>MQRADSEQPSKRPRCDDSPRTPSNTPSAEADWSPGLELHPDYKTWGPEQVCSFLRRGGFEEPVLLKNIRENEITGALLPCLDESRFENLGVSSLGERKKLLSYIQRLVQIHVDTMKVINDPIHGHIELHPLLVRIIDTPQFQRLRYIKQLGGGYYVFPGASHNRFEHSLGVGYLAGCLVHALGEKQPELQISERDVLCVQIAGLCHDLGHGPFSHMFDGRFIPLARPEVKWTHEQGSVMMFEHLINSNGIKPVMEQYGLIPEEDICFIKEQIVGPLESPVEDSLWPYKGRPENKSFLYEIVSNKRNGIDVDKWDYFARDCHHLGIQNNFDYKRFIKFARVCEVDNELRICARDKEVGNLYDMFHTRNSLHRRAYQHKVGNIIDTMITDAFLKADDYIEITGAGGKKYRISTAIDDMEAYTKLTDNIFLEILYSTDPKLKDAREILKQIEYRNLFKYVGETQPTGQIKIKREDYESLPKEVASAKPKVLLDVKLKAEDFIVDVINMDYGMQEKNPIDHVSFYCKTAPNRAIRITKNQVSQLLPEKFAEQLIRVYCKKVDRKSLYAARQYFVQWCADRNFTKPQDGDVIAPLITPQKKEWNDSTSVQNPTRLREASKSRVQLFKDDPM[4x]

Sterile alpha motif and HD-domain containing protein 1 (SAMHD1) is a dNTP triphosphohydrolase that catalyses the breakdown of dNTPs to constituent 2′-deoxynucleoside and triphosphate, and is therefore an important regulator of cellular nucleotide homeostasis in mammalian cells. SAMHD1 dNTP triphosphohydrolase catalytic activity requires assembly into homo-tetramers. Sequences at the N- and C-termini of the HD domain stabilise inter-monomer protein-protein interactions and incorporate four pairs of allosteric, AL1 and AL2, nucleotide-binding sites. Nucleotide binding at these sites promote tetramer-assembly and regulate SAMHD1 through combined binding of G-based (AL1) and 2’-deoxynucleoside (AL2) triphosphates.

The State-III C2 tetramer, AC Dimer-2 is further relaxed with more disordered C-terminal lobe- linkers, active sites are exposed and empty. BD Dimer-2 retains the tense state with substrate-loaded active sites, all allosteric sites are occupied. d The depletion phase, States-IV and -V predominate. In State-III, the active sites of the tense side of the tetramer also maintain the same nucleotide configuration as in State-I and State-II. However, the active sites on the relaxed side are now completely empty with no substrate or products bound. Further examination of the nucleotide content reveals that on the tense side, in both State-II and State-III tetramers, the active sites contain substrate dNTPs, and the allosteric sites are loaded with GTP-dNTP pairs. In State-III the further movement of the C-terminal lobes away from the lobe-linkers results in loss of all remaining interactions constituting a released conformation.>MKVLGVVVEYNPFHNGHLYHLTSARELVKPDYTIAVMSGNFCQRGEPAVIDKFARAEIALRMGVDVVLELPVVFATQDAGGFAFGAVCVLDATGVVTDVVFGSESNDIEFLQRVARILYEQPDEYQKFLHEELKKGYSFPNARKYALMRYFSMKGWNEEEVLKLEKSNDILGVEYIHSALKIGSNIRFHTIKRVGAEEKDTSFRGRFSSATAIRNLMREKRWEEVRDSLPEDSFEILMREINEGRGPVFLENMGDFLLSFFRLKNMDFFEKIHGFSEGLEKRFHVCARQTGSYRDFLECVKAKRFTFSRIRRLALFSVFEVNKEFVEKSN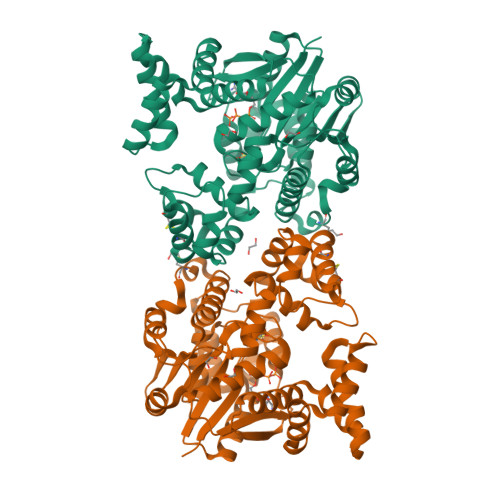TKGPQYIRILGFTEKGREILSLMRKKAKLPIVTNMSLYRKVLEKTDLPVDKQLFLEQIDLDVKATNFYSMFFPSVEQRCGERDFSIHPIFLRTEM[4x]> ADQRRDFIDIESKFALRTPEDTAEDTCHLIPGVAESVATCHFNHSSKTFMVIHGWTVTGMYESWVPKLVAALYKREPDSNVIVVDWLSRAQEHYPVSAGYTKLVGQDVARFINWMEEEFNYPLDNVHLLGYSLGAHAAGIAGSLTNKKVNRITGLDPAGPNFEYAEAPSRLSPDDADFVD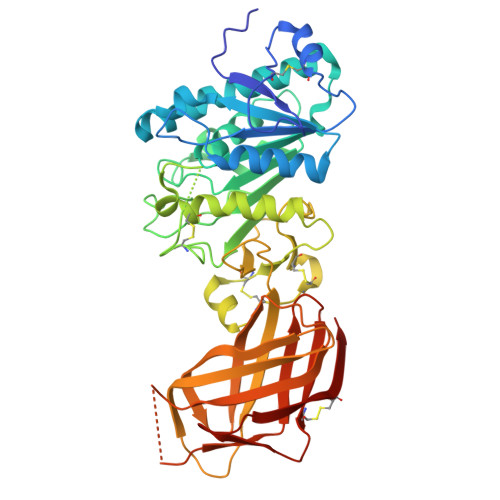VLHTFTRGSPGRSIGIQKPVGHVDIYPNGGTFQPGCNIGEAIRVIAERGLGDVDQLVKCSHERSIHLFIDSLLNEENPSKAYRCSSKEAFEKGLCLSCRKNRCNNLGYEINKVRAKASSKMYLKTRSQMPYKVFHYQVKIHFSGTESETHTNQAFEISLYGTVAESENIPFTLPEVSTNKTYSFLIYTEVDIGELLMLKLKWKSDSYFSWSDWWSSPGFAIQKIRVKAGETQKKVIFCSREKVSHLQKGKAPAVFVKCHDKSLNKKSG>VRERGPQRVAAHITGTRGRSNTLSSPNSKNEKALGRKINSWESSRSGHSFLSNLHLRNGELVIHEKGFYYIYSQTYFRFQEEIKENTKNDKQMVQYIYKYTSYPDPILLMKSARNSCWSKDAEYGLYSIYQGGIFELKENDRIFVSVTNEHLIDMDHEASFFGAFLVG[3x];>[3x]ALITQQDLAPQQRAAPQQKRSSPSEGLCPPGHHISEDGRDCISCKYGQDYSTHWNDLLFCLRCTRCDSGEVELSPCTTTRNTVCQCE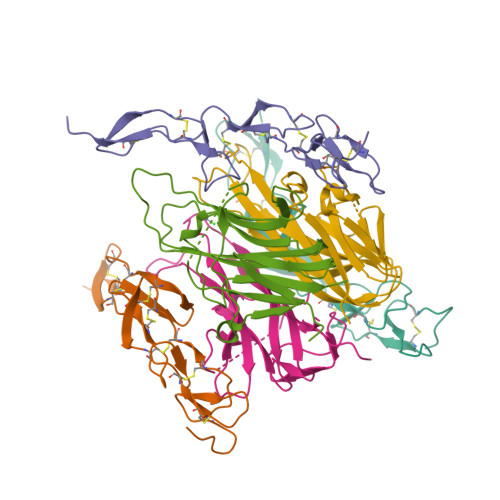EGTFREEDSPEMCRKCRTGCPRGMVKVGDCTPWSDIECVHKES>MSELSEIDSVAGVTIYSVDGEPKSFVYKAGFAIDADGAPNAYAPNNGGTDFTANGGDDQGGDWWGGPVDAEGYPIKQKIFDPFPGYYVSATAHFNPAYSEDSPYRYIDSNSIPFIVLPGNHSNGAKLGDVALVYNEKTGDNCYAIYGDVGPSSKIGEGSVRLAQALKIDDNPKAGGTESRIVVTLVFPGSVGKWETPKRWFSHANQLTKAWGGLSRLKTLSDQL[2x]

We focus on AMGs that potentially encode chitosanase enzymes that metabolize chitin – a common carbon polymer. One expressed protein showing endo-chitosanase activity (V-Csn) is crystalized and structurally characterized at ultra-high resolution, thus representing the structure of a soil viral AMG product. The structure consisted of two non-contiguous structural domains. Our rigorous analyses not only resulted in a crystal structure of a soil viral AMG product, but also enabled us to propose the mode of action of this previously uncharacterized chitosanase enzyme in the GH75 family of glycosyl hydrolases.

The V-Csn structure was solved in two crystal forms; apo1 containing a single molecule in the asymmetric unit, and apo2 containing a dimer in the asymmetric unit. The apo2 crystal form was solved by molecular replacement using the refined apo1 structure as the search model, and refined with phenix.refine. The apo2 structure has two independent V-Csn molecules in the asymmetric unit and the two molecules form a non-crystallographic dimer. Superposition of the two molecules of the apo2 dimer onto the apo1 structure gives a root-mean-squared deviation (RMSD) of 0.45 Å for both molecules. In the apo1 crystal form, the same dimer is observed albeit generated by the crystallographic symmetry of the C2 space group. This is consistent with the observation that V-Csn exists as a dimer in solution based on size exclusion chromatography, although there is no evidence that dimerization is required for enzyme activity. Formation of the dimer buries 1830 Å2 (∼9%) of the surface per monomer. The regions of contact involve the loop between β-strands β4 and β5 (in Domain-2) in one molecule slotting between helices α3 and α4 in the second molecule, linked via hydrogen bonding and hydrophobic interactions with residues from the two helices and strand β8.The nuclear retinoid X receptor (RXR) is a unique family of ligand-activated transcription factors, which in humans comprises of three members, namely, RXRα (NR2B1), RXRβ (NR2B2) and RXRγ (NR2B3). All three RXR isoforms typically function as a universal heterodimer partner for other nuclear receptors, including the type II thyroid hormone receptors (THRs, NR1A1-2) and the peroxisome proliferator-activated receptors (PPARs, NR1C1-3). Here, we report a complete set of the crystal structures for all three RXR isoforms in active, ligand-bound conformation with an identical ligand. In addition, we discovered saturated fatty acids, including palmitic acid (PA), myristic acid (MA) and stearic acid (SA), as RXR modulators capable of inducing the recruitment of co-regulators to the RXR ligand-binding domain (LBD) and hence, activating the receptor.

We next questioned whether PA could also bind to the other two RXR isoforms and therefore, we crystallized and successfully determined the tertiary complex structures of both RXRβ and RXRγ with (exogenously added) PA and the GRIP-1 co-regulator peptide. The crystal structures indeed revealed the binding of PA to both isoforms in a similar manner to that observed for the alpha counterpart. Overall, binding of PA induced similarly an active state of RXRα, RXRβ and RXRγ. The three structures were highly identical, supported by the superimposition root-mean-square deviation of atomic positions (RMSD) of 0.29 Å. A detailed structural analysis showed that PA occupied identically the canonical ligand-binding site and engaged in similar interactions in all three RXR isoforms. No conformational changes were observed for the residues lining the pocket. We observed that none of those amino acid differences were lining the ligand-binding pocket, confirming previous assumptions that the RXR ligand-binding sites are conserved. To understand whether the 24 amino acid differences within the LBD region may have any indirect influence toward ligand-binding properties among the three isoforms, we mapped the differences onto the structures. We observed that although most changes were located peripherally at the surface of the proteins, there were three substitutions in the proximity of the ligand-binding pocket (site 3, site 11 and site 15 based on Figure 4a). Among them, a minor difference in the lipophilic residue at site 15 (α: Val374, β: Ile445, γ: Val375) located in helix 8 might affect interactions between helices 5 and 8. Since helix 5 is involved in ligand-binding site formation, this difference could allow contributions to subtype preference through differential ability of helix 5 movement in the RXR isoforms.

> SMEMPVDRILEAELAVEQKSDQGVEGPGGTGGSGSSPNDPVTNICQAADKQLFTLVEWAKRIPHFSSLPLDDQVILLRAGWNELLIASFSHRSIDVRDGILLATGLHVHRNSAHSAGVGAIFDRVLTELVSKMRDMRMDKTELGCLRAIILFNPDAKGLSNPSEVEVLREKVYASLETYCKQKYPEQQGRFAKLLLRLPALRSIGLKCLEHLFFFKLIGDTPIDTFLMEMLEAPHQLA;> KHKILHRLLQDSSY> DDYLDRLPKSKKGLQGLLQDIEKRILHYKQLFFKEQNEIANGKRSMVPDNSIPICSDVTKLNFQALIDAQMRHAGKMF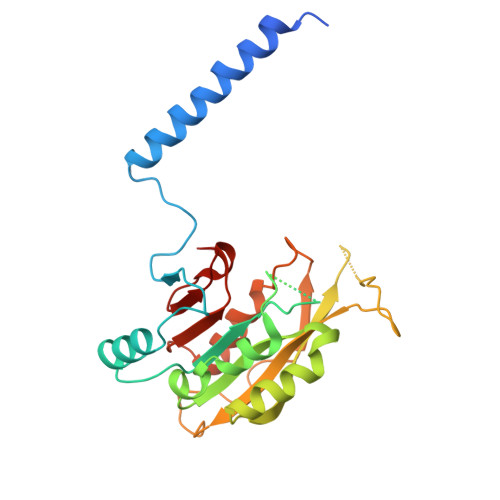DVIMMDPPWQLSSSQPSRGVAIAYDSLSDEKIQNMPIQSLQQDGFIFVWAINAKYRVTIKMIENWGYKLVDEITWVKKTVNGKIAKGHGFYLQHAKESCLIGVKGDVDNGRFKKNIASDVIFSERRGQSQKPEEIYQYINQLCPNGNYLEIFARRNNLHDNWVSIGNEL>MPRQASTFTNPVLWEDHPALEVFRVGSVFYYSSSTFAYSPGAPVLKSYDLVHWTPVTHSVPRLNFGSNYDLPSGTPGAYVKGIWASTLRYRRSNDRFYWYGCVEGRTYLWTSPGGNALANNGEVPPSAWNWQHTATIDNCYYDAGLLIDDDDTMYIAYGNPTINVAQLSPDGTRQVRVQQRVYAHPQGQTVEGARMYKIRGNYYILVTRPADAEYVLRSTTGSPFGPYEARTLVSRIQGPLANAGFAHQGGIVDAPDGTWHYVAFMDAYPGGRIPVVAPLRWTADGWPEVVTDSQGRWGTSYPIPVRGAKNATEGLASTDLDEFRGTRFSEHWEWNHNPDTSKFTLLGGNEGGLILRTATVTGDLFAARNTLTRRIAGPKASGIFRLDVRGMRDGDR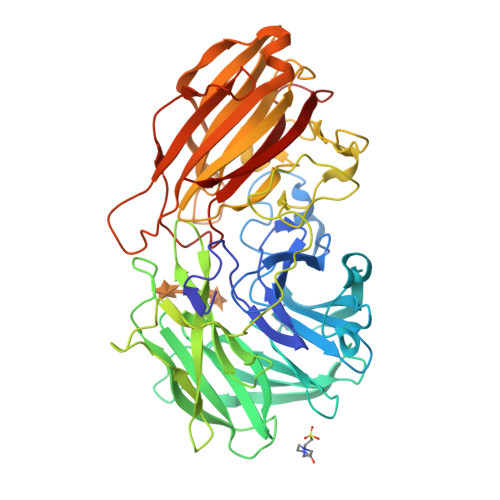AGAVLFRDRAAYIGVWKQGNEARIVMVDDLRLNEDGWRTASTGRVAANGPVIDTNAQQDIWLRIDADITPAFGTNTERTTTFYYSIDGGRTYTRLGPAFAMTNSWRYFTGYRFGVFNFSTKSLGGEVKVKGFKMNMILEHHHHHH[2x]> MDKLFSMIEVEVNSQCNRTCWYCPNSVSKRKETGEMDPALYKTLMEQLSSLDFAGRISFHFYGEPLLC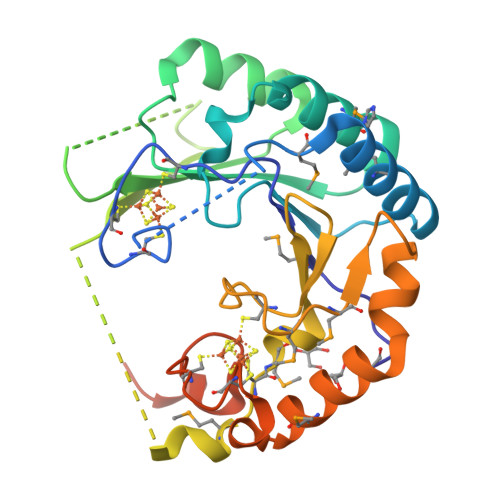KNLDLFVGMTTEYIPRARPIIYTNGDFLTEKRLQTLTELGIQKFIVTQHAGAKHKFRGVYDQLAGADKEKVVYLDHSDLVLSNRGGILDNIPQASKANMSCMVPSNLAVVTVLGNVLPCFEDFNQKMVMGNIGEQHISDIWHNDKFTSFRKMLKEGHRGKSDLCKNCNNVSVQTEEQYDYVLNSSSVDKLAAALEHHHHHH>MSGTKPDILWAPHHVDRFVVCDSELSLYHVESTVNSELKAGSLRLSEDSAATLLSINSDTPYMKCVAWYLNYDPECLLAVGQANGRVVLTSLGQDHNSKFKDLIGKEFVPKHARQCNTLAWNPLDSNWLAAGLDKHRADFSVLIWDICSKYTPDIVPMEKVKLSAGETETTLLVTKPLYELGQNDACLSLCWLPRDQKLLLAGMHRNLAIFDLRNTSQKMFVNTKAVQGVTVDPYFHDRVASFYEGQVAIWDLRKFEKPVLTLTEQPKPLTKVAWCPTRTGLLATLTRDSNIIRLYDMQHTPTPIGDETEPTIIERSVQPCDNYIASFAWHPTSQNRMIVVTPNRTMSDFTVFERISLAWSPITSLMWACGRHLYECTEEENDNSLEKDIATKMRLRALSRYGLDTEQVWRNHILAGNEDPQLKSLWYTLHFMKQYTEDMDQKSPGNKGSLVYAGIKSIVKSSLGMVESSRHNWSGLDKQSDIQNLNEERILALQLCGWIKKGTDVDVGPFLNSLVQEGEWERAAAVALFNLDIRRAIQILNEGASSEKGDLNLNVVAMALSGYTDEKNSLWREMCSTLRLQLNNPYLCVMFAFLTSETGSYDGVLYENKVAVRDRVAFACKFLSDTQLNRYIEKLTNEMKEAGNLEGILLTGLTKDGVDLMESYVDRTGDVQTASYCMLQGSPLDVLKDERVQYWIENYRNLLDAWRFWHKRAEFDIHRSKLDPSSKPLAQVFVSCNFCGKSISYSCSAVPHQGRGFSQYGVSGSPTKSKVTSCPGCRKPLPRCALCLINMGTPVSSCPGGTKSDEKVDLSKDKKLAQFNNWFTWCHNCRHGGHAGHMLSWFRDHAECPVSACTCKCMQLDTTGNLVPAETVQP[4x];>MEKMSRVTTALGGSVLTGRTMHCHLDAPANAISVCRDAAQVVVAGRSIFKIYAIEEEQFVEKLNLRVGRKPSLNLSCADVVWHQMDENLLATAATNGVVVTWNLGRPSRNKQDQLFTEHKRTVNKVCFHPTEAHVLLSGSQDGFMKCFDLRRKDSVSTFSGQSESVRDVQFSIRDYFTFASTFENGNVQLWDIRRPDRCERMFTAHNGPVFCCDWHPEDRGWLATGGRDKMVKVWDMTTHRAKEMHCVQTIASVARVKWRPECRHHLATCSMMVDHNIYVWDVRRPFVPAAMFEEHRDVTTGIAWRHPHDPSFLLSGSKDSSLCQHLFRDASQPVERANPEGLCYGLFGDLAFAAKESLVAAESGRKPYTGDRRHPIFFKRKLDPAEPFAGLASSALSVFETEPGGGGMRWFVDTAERYALAGRPLAELCDHNAKVARELGRNQVAQTWTMLRIIYCSPGLVPTANLNHSVGKGGSCGLPLMNSFNLKDMAPGLGSETRLDRSKGDARSDTVLLDSSATLITNEDNEETEGSDVPADYLLGDVEGEEDELYLLDPEHAHPEDPECVLPQEAFPLRHEIVDTPPGPEHLQDKADSPHVSGSEADVASLAPVDSSFSLLSVSHALYDSRLPPDFFGVLVRDMLHFYAEQGDVQMAVSVLIVLGERVRKDIDEQTQEHWYTSYIDLLQRFRLWNVSNEVVKLSTSRAVSCLNQASTTLHVNCSHCKRPMSSRGWVCDRCHRCASMCAVCHHVVKGLFVWCQGCSHGGHLQHIMKWLEGSSHCPAGCGHLCEYS[2x];>[2x]MAARWSSENVVVEFRDSQATAMSVDCLGQHAVLSGRRFLYIVNLDAPFEGHRKISRQSKWDIGAVQWNPHDSFAHYFAASSNQRVDLYKWKDGSGEVGTTLQGHTRVISDLDWAVFEPDLLVTSSVDTYIYIWDIKDTRKPTVALSAVAGASQVKWNKKNANCLATSHDGDVRIWDKRKPSTAVEYLAAHLSKIHGLDWHPDSEHILATSSQDNSVKFWDYRQPRKYLNILPCQVPVWKARYTPFSNGLVTVMVPQLRRENSLLLWNVFDLNTPVHTFVGHDDVVLEFQWRKQKEGSKDYQLVTWSRDQTLRMWRVDSQMQRLCANDILDGVDEFIESISLLPEPEKTLHTEDTDHQHTASHGEEEALKEDPPRNLLEERKSDQLGLPQTLQQEFSLINVQIRNVNVEMDAADRSCTVSVHCSNHRVKMLVKFPAQYPNNAAPSFQFINPTTITSTMKAKLLKILKDTALQKVKRGQSCLEPCLRQLVSCLESFVNQEDSASSNPFALPNSVTPPLPTFARVTTAYGSYQDANIPFPRTSGARFCGAGYLVYFTRPMTMHRAVSPTEPTPRSLSALSAYHTGLIAPMKIRTEAPGNLRLYSGSPTRSEKEQVSISSFYYKERKSRRWKSKREGSDSGNRQIKAAGKVIIQDIACLLPVHKSLGELYILNVNDIQETCQKNAASALLVGRKDLVQVWSLATVATDLCLGPKSDPDLETPWARHPFGRQLLESLLAHYCRLRDVQTLAMLCSVFEAQSRPQGLPNPFGPFPNRSSNLVVSHSRYPSFTSSGSCSSMSDPGLNTGGWNIAGREAEHLSSPWGESSPEELRFGSLTYSDPRERERDQHDKNKRLLDPANTQQFDDFKKCYGEILYRWGLREKRAEVLKFVSCPPDPHKGIEFGVYCSHCRSEVRGTQCAICKGFTFQCAICHVAVRGSSNFCLTCGHGGHTSHMMEWFRTQEVCPTGCGCHCLLESTF;>MFVARSIAADHKDLIHDVSFDFHGRRMATCSSDQSVKVWDKSESGDWHCTASWKTHSGSVWRVTWAHPEFGQVLASCSFDRTAAVWEEIVGESNDKLRGQSHWVKRTTLVDSRTSVTDVKFAPKHMGLMLATCSADGIVRIYEAPDVMNLSQWSLQHEISCKLSCSCISWNPSSSRAHSPMIAVGSDDSSPNAMAKVQIFEYNENTRKYAKAETLMTVTDPVHDIAFAPNLGRSFHILAIATKDVRIFTLKPVRKELTSSGGPTKFEIHIVAQFDNHNSQVWRVSWNITGTVLASSGDDGCVRLWKANYMDNWKCTGILKGNGSPVNGSSQQGTSNPSLGSTIPSLQNSLNGSSAGRKHS[6x];>MVSVINTVDTSHEDMIHDAQMDYYGTRLATCSSDRSVKIFDVRNGGQILIADLRGHEGPVWQVAWAHPMYGNILASCSYDRKVIIWREENGTWEKSHEHAGHDSSVNSVCWAPHDYGLILACGSSDGAISLLTYTGEGQWEVKKINNAHTIGCNAVSWAPAVVPGSLIDHPSGQKPNYIKRFASGGCDNLIKLWKEEEDGQWKEEQKLEAHSDWVRDVAWAPSIGLPTSTIASCSQDGRVFIWTCDDASSNTWSPKLLHKFNDVVWHVSWSITANILAVSGGDNKVTLWKESVDGQWVCISDVNKGQGSVSASVTEGQQNEQ[2x];>[2x]MELHILEHRVRVLSVARPGLWLYTHPLIKLLFLPRRSRCKFFSLTETPEDYTLMVDEEGFKELPPSEFLQVAEATWLVLNVSSHSGAAVQAAGVTKIARSVIAPLAEHHVAVLMLSTYQTDFILVREQDLSVVIHTLAQEFDIYREVGGEPVPVTRDDSSNGFPRTQHGPSPTVHPIQSPQNRFCVLTLDPETLPAIATTLIDVLFYSHSTPKEAASSSPEPSSITFFAFSLIEGYISIVMDAETQKKFPSDLLLTSSSGELWRMVRIGGQPLGFDECGIVAQIAGPLAAADISAYYISTFNFAHALVPEDGIGSVIEVLQRRQEGLAS

Mechanistic target of rapamycin complex 1 (mTORC1) is a nutrient-responsive master regulator of metabolism. Under low nutrients, including arginine, the GTPase-activating protein complex GATOR1 promotes GTP hydrolysis on RagA/B, inactivating mTORC1. GATOR1 is regulated by the cage-like GATOR2 complex and cytosolic amino acid sensors. Instead, a series of dedicated amino acid sensors that include CASTOR1, sestrin2 (SESN2) and SAMTOR relay information about amino acids into the pathway through the intermediation of the GATOR1–GATOR2–KICSTOR complexes.

To understand how the arginine sensor CASTOR1 binds to GATOR2 to disinhibit GATOR1 under low cytosolic arginine, we determined the cryo-electron microscopy structure of human GATOR2 bound to CASTOR1 in the absence of arginine. The purified GATOR2 and CASTOR1apo were combined and the cryo-electron microscopy (cryo-EM) structure of GATOR2 bound to CASTOR1apo was determined to an overall resolution of 3.89 Å. In the GATOR2-bound structure, a single CASTOR1apo homodimer binds across one face of the GATOR2 cage, engaging one MIOS β-propeller domain per CASTOR1apo monomer. The two MIOS subunits straddling the ‘front’ face of GATOR2 engage the CASTOR1 homodimer, while the other two back-facing MIOS β-propellers that do not engage CASTOR1 are disordered and are not seen in the final density map and reconstruction. Specifically, upon interaction with CASTOR1, the front-face MIOS β-propeller pair breaks the internal interface, pushing 10 Å apart and rotating by 16° relative to the MIOS α-solenoid domains of the inner core of the GATOR2 cage In the GATOR2 unbound conformation, the MIOS interface responsible for interaction with CASTOR1 is exposed and not buried in the β-propeller interface. Compared to GATOR2apo, this movement in the front-face MIOS α-solenoid and CTD domains results in the disordering of residues 757–836 and 890–921 in WDR59 and residues 727–746 and 770–783 in MIOS. Two MIOS loops are responsible for most of the contacts with CASTOR1apo. The MIOS loops contacts are centered on the basic residues H112, H136 and R137, with K135 at the edge of the contact region. These four basic residues engage with a complementary electronegative pocket on the surface of CASTOR1apo centered on D121 and also containing Y118, Q119 and Y236. In CASTOR1apo, the MIOS-releasing loop is disordered, which exposes the negatively charged MIOS-binding interface residues Y118, Q119, D121 and Y236. In the CASTOR1Arg structure, residues 90–94 in the MIOS-releasing loop are ordered, cover the MIOS-binding interface and sterically block the MIOS–CASTOR1 interaction.> XRTWEEWDRA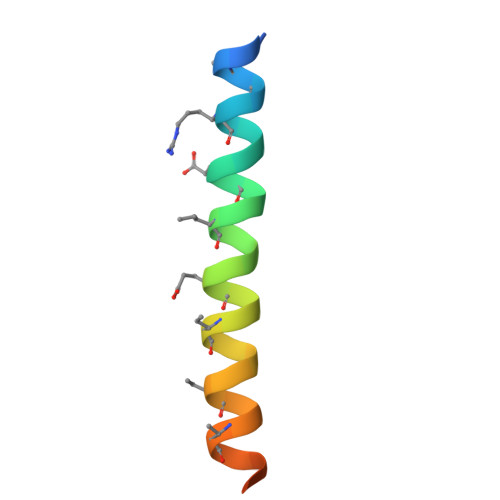IAEYARRIEELIRAAQEQQRKNEEALREL>VDFHGYARSGIGWTGSGGEQQCFQATGAQSKYRLGNECETYAELKLGQEVWKEGDKSFYFDTNVAYSVNQQNDWESTDPAFREANVQGKNLIEWLPGSTIWAGKRFYQRHDVHMIDFYYWDISGPGAGIENIDLGFGKLSLAATRSTEAGGSYTFSSQNIYDEVKDTANDVFDVRLAGLQTNPDGVLELGVDYGRANTTDGYKLADGASKDGWMFTAEHTQSMLKGYNKFVVQYATDAMTTQGKGQARGSDGSSSFTEELSDGTKINYANKVINNNGNMWRILDHGAISLGDKWDLMYVGMYQNIDWDNNLGTEWWTVGVRPMYKWTPIMSTLLEVGYDNVKSQQTGDRNNQYKITLAQQWQAGDSIWSRPAIR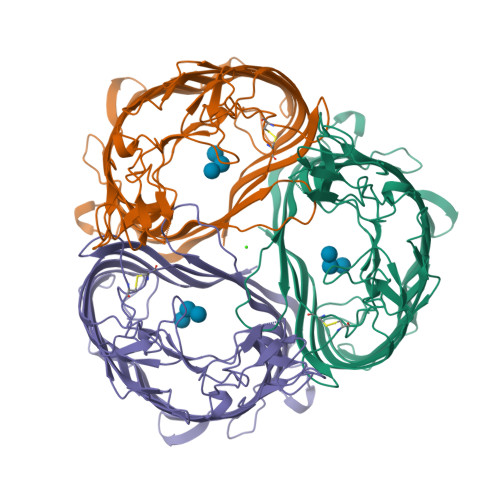IFATYAKWDEKWGYIKDGDNISRYAAATNSGISTNSRGDSDEWTFGAQMEIWW[3x]Different AAF variants are expressed by different EAEC strains, where they are required for the bacterium's adherence to small and large intestinal mucosa. As with Afa/Dr polyadhesins, AAF consist of two secreted protein subunits, a major subunit (A) and a putative minor subunit (B). In the fiber, subunits are linked together by donor strand complementation (DSC) with an N-terminal Gd donor strand segment of one subunit inserted into the hydrophobic cleft of a neighboring subunit. In this study, we report X-ray crystallographic and NMR studies of monomeric, donor-strand-complemented major and minor subunits of AAF/I from the German outbreak strain and AAF/II from EAEC strain 042 and provide an atomic resolution model for the structure of the entire fimbriae.

In EAEC, the minor subunit of AAF/II (AafB) has been associated with the release of cytokines, suggesting its surface localization and function in EAEC pathogenesis. At the same time, based on the fact that minor subunits of AAF are 12–23 residues shorter than major subunits, we hypothesized that they do not possess their own donor strand sequences and are stabilized in the fiber by strands donated by major subunits. The minor subunits AggBdsA and AafBdsA have more similar structures than the major pilins: 117 matching Cα atoms are superimposed with r.m.s.d. of 1.2 Å. The donor sequences derived from the corresponding major subunits form classical donor strands (Gd), each inserting five donor residues into the subunit core structure. The values of shape correlation statistic (Sc) calculated for the acceptor cleft-donor strand interactions for AggBdsA and AafBdsA (0.733 and 0.756, respectively) were similar to those calculated for AggAdsA and AafAdsA (0.784 and 0.804, respectively). The good geometrical fit between the donor strands and acceptor clefts suggests that these interactions are native. As predicted, the minor subunits have no N-terminal extension that could act as a donor strand: the first residue in the mature protein is structured and immediately followed by the first strand A. Hence, this structural evidence suggests that the minor subunits assemble by accepting donor sequences of the corresponding major subunits. As such sequences are only available in tip subunits of major subunit polymers, the AAF minor subunits are likely to be tip localized. In minor subunits, strand A is not split between the β sheets, but locates entirely in the sheet 1. Instead, strand C2 that in a classical Ig fold is hydrogen bonded to strand F, in minor subunits is hydrogen bonded to strand D and hence belongs to sheet 2.

>MRGSHHHHHHGSTEISLEGLHRNMGEQLFDGDILATGRIICRERHTGFHIQMNARQVEGRPGHYIVQGSKDTQSKLWVRLGREGWTSPTGGGQQGIVRSGQEEQVIFDVMADGNQWAKPGEYIFSVSGKCLTSWEDNKQNATAVAKTATSTITVV[2x]>[2x]MNGPIIMTREERMKIVHEIKERILDKYGDDVKAIGVYGSLGRQTDGPYSDIEMMCVMSTEEAEFSHEWTTGEWKVEVNFDSEEILLDYASQVESDWPLTHGQFFSILPIYDSGGYLEKVYQTAKSVEAQTFHDAICALIVEELFEYAGKWRNIRVQGPTTFLPSLT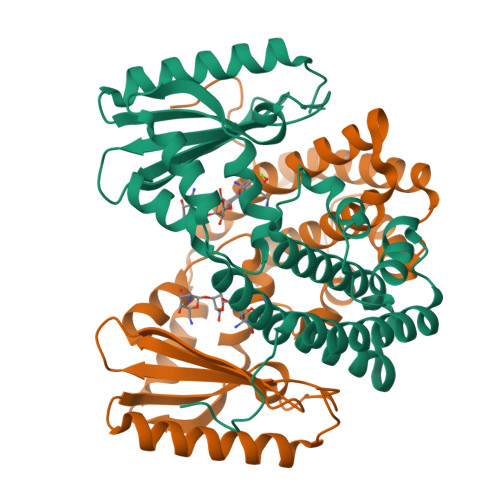VQVAMAGAMLIGLHHRICYTTSASVLTEAVKQSDLPSGYDHLCQFVMSGQLSDSEKLLESLENFWNGIQEWTERHGYIVDVSKRIPF> GPL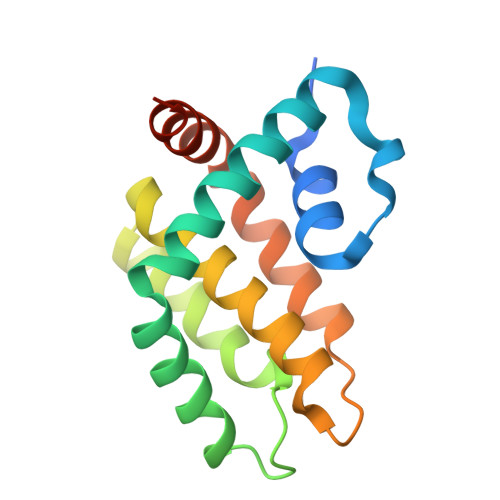GSMDNCNYNIEKVLNVYLRDLRIESLNNNELEILIMIRECCEVIKKDYKTEFNEICNFILQNNVKSCYDINDVKNIIIETINSDFRPSVILASISLLSIIIKKKKDENNEVVDDDLALNELINKFSSYQKDIISFVEKNKKKNKQND>[4x]MSILHMPLKIKDITIKNRIMMSPMCMYSASTDGMPNDWHIVHYATRAIGGVGLIMQEATAVESRGRITDHDLGIWNDEQVKELKKIVDICKANGAV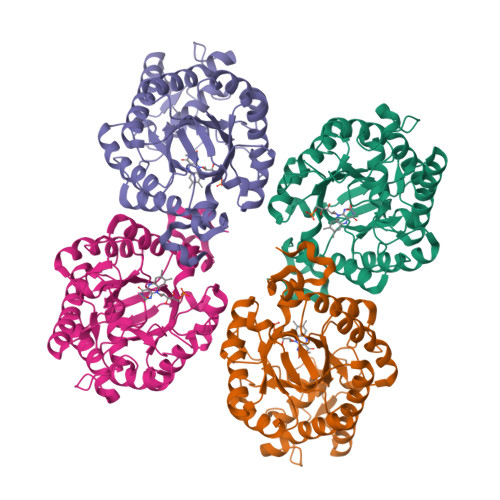MGIQLAHAGRKCNISYEDVVGPSPIKAGDRYKLPRELSVEEIKSIVKAFGEAAKRANLAGYDVVEIHAAHGYLIHEFLSPLSNKRKDEYGNSIENRARFLIEVIDEVRKNWPENKPIFVRVSADDYMEGGINIDMMVEYINMIKDKVDLIDVSSGGLLNVDINLYPGYQVKYAETIKKRCNIKTSAVGLITTQELAEEILSNERADLVALGRELLRNPYWVLHTYTSKEDWPKQYERAFKKHHHHHH> MGHHHHHHHHHHSSHIEGRHMQELFNNLMELCKDSQRKFFYSDDVSASGRTYRIFSYNYASYSDWLLPDALECRGIMFEMDGEKPVRIASRPMEKFFNLNENPFTMNIDLNDVDYILTMEDGSLVSTYLDGDEILFKSKGSIKSEQALMANGILMNINHHRLRDRLKELAEDGFTANFEFVAPTNRIVLAYQEMKIILLNVRENETGEYISYDDIY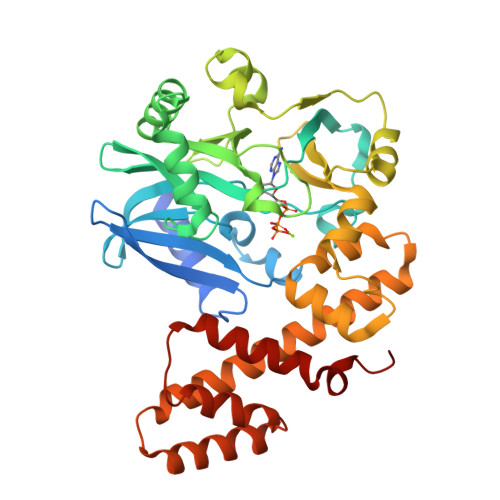KDATLRPYLVERYEIDSPKWIEEAKNAENIEGYVAVMKDGSHFKIKSDWYVSLHSTKSSLDNPEKLFKTIIDGASDDLKAMYADDEYSYRKIEAFETTYLKYLDRALFLVLDCHNKHCGKDRKTYAMEAQGVAKGAGMDHLFGIIMSLYQGYDSQEKVMCEIEQNFLKNYKKFIPEGY>ASDASPIAYVNLPQAFVFNVTGDSRDRLVQIKAQLMVRGAENEELARYHSPLIESSLLSTFASATVDQLRSPTGRVELRDRASEDIKAALNAAVGKPVIEKVLFTDFVIQ[2x]

FliL, a component protein of the flagellar motor, is known to enhance the motor performance under high-load conditions in some bacteria. A flagellar protein, FliL, which is a single-transmembrane protein with a large periplasmic region and associates with the flagellar basal body, has been found to be important for the function of the motor under high-load conditions, such as the highly viscous environments in some species. Polar FliL is composed of an N-terminal short cytoplasmic region (residues 1 to 17), a single transmembrane region (TM) (residues 18 to 40), and a periplasmic region (FliLPeri) (residues 41 to 167). FliLPeri shows a remarkable structural similarity to the stomatin/prohibitin/flotillin/HflK/C (SPFH) domain of stomatin family proteins, some of which are involved in modulation of ion channel activities in various organisms.

FliLPeri was immediately digested into a fragment composed of residue 58 to 167 that is named FliLC, and FliLC is highly resistant to trypsin digestion. Thus, we concluded that FliLC is a core region of FliLPeri and that the N-terminal 17 residues (residues 41 to 58; FliLL) act as a linker connecting the TM region with FliLC. The FliLC crystal belongs to the space group of P61 and contains two molecules in an asymmetric unit. FliLC consists of a single domain with a bean shape containing four α-helices (α1 to α4) and one β-sheet composed of four β-strands (β1 to β4). The β-sheet is highly twisted at the middle and therefore can be divided in two subsheets, subsheet 1 (S1) and S2. S1 consists of β1, β3, and β4, and S2 is composed of β2, β3, and β4. The two molecules in the asymmetric unit of the FliLC crystal are related by 30° rotation around the crystallographic 61 screw axis with a translation of 1/12 of the repeat along the c axis; thus, the molecules form a helical tube with 121 screw symmetry along the c axis in the FliLC crystal. The neighboring subunit in the FliLC crystal is slightly tilted compared with that in the FliLPeri ring, resulting in the formation of the helical tube rather than the ring. The interaction between the subunits related by the 121 screw symmetry is almost the same as that in the FliLPeri ring except for the lack of hydrogen bonds between T162 and Q71 and between D163 and V74. FliLC shows remarkable structural similarity to the SPFH domain despite the low similarity of amino acid sequence.> MSRLDKSKVINSALELLNEVGIEGLTTRKLAQKLGVEQPTLYWHVKNKRALLDALAIEMLDRHHTHFSPLEGESWQDFLRNNAKSFRNALLSHRDGAKVHLGTRPTEKQYETLENQLA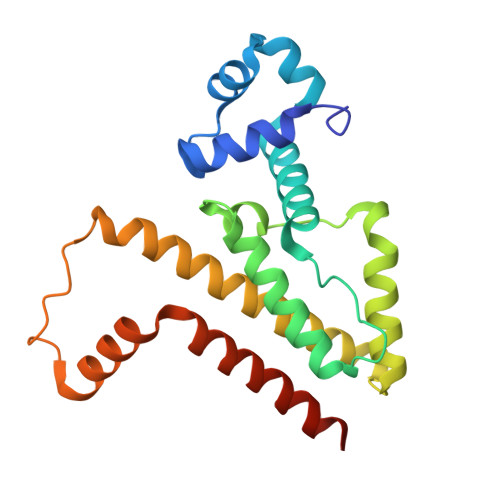FLTQQGFSLENALYALSAVGHFTLGSVLEDQEHQVAKEERETPTTDSMPPLLRQAIELFDHQGAEPAFLHGLESLIRGFEVQLTALLQIV> MDSQRNLLVIALLFVSFMIWQAWEQDKNPQPQAQQTTQTTTTAAGSAADQGVPASGQGKLISVKTDVLDLTINTRGGDVEQALLPAYPKELNSTQPFQLLETSPQFIYQAQSGLTGRDGPDNPANGPRPLYNVEKDAYVLAEGQNELQVPMTYTDAAGNTFTKTFVLKRGDYAVNVNYNVQNAGEKPLEISTFGQLKQSITLPPHLDTGSSNFALHTFRGAAYSTPDEKYEKYKFDTIADNENLNISSKGGWVAMLQQYFATAWIPHNDGTNNFYTANLGNGIAAIGYKSQPVLVQPGQTGAMNSTLWVGPEIQDKMA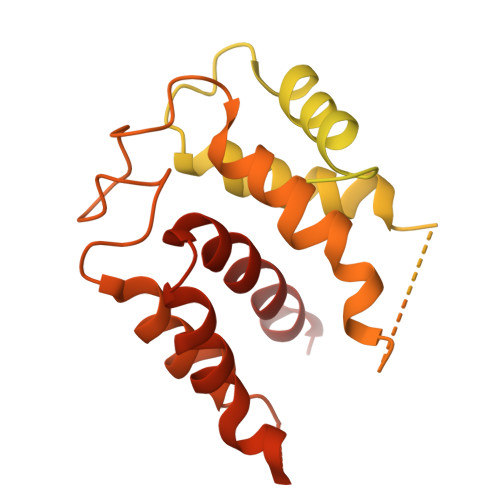AVAPHLDLTVDYGWLWFISQPLFKLLKWIHSFVGNWGFSIIIITFIVRGIMYPLTKAQYTSMAKMRMLQPKIQAMRERLGDDKQRISQEMMALYKAEKVNPLGGCFPLLIQMPIFLALYYMLMGSVELRQAPFALWIHDLSAQDPYYILPILMGVTMFFIQKMSPTTVTDPMQQKIMTFMPVIFTVFFLWFPSGLVLYYIVSNLVTIIQQQLIYRGLEKRGLLESSGENLYFQ> MTYKYNCCDDGSGTTVGSVVRFDNVTLLIDPGWNPSKVSYEQCIKYWEKVIPEIDVIILSQPTIECLGAHSLLYYNFTSHFISRIQVYATLPVINLGRVSTIDSYASAGVIGPYDTNKLDLEDIEISFDHIVPLKYSQLVDLRSRYDGLTLLAYNAGVCPGGSIWCISTYSEKLVYAKRWNHTRDNILNAASILDATGKPLSTLMRPSAIITTLDRFGSSQPFKKRSKIFKDTLKKGLSSDGSVIIPVDMSGKFLDLFTQVHELLFESTKINAHTQVPVLILSYARGRTLTYAKSMLEWLSPSLLKTWENRNNTSPFEIGSRIKIIAPNELSKYPGSKICFVSEVGALINEVIIKVGNSEKTTLILTKPSFECASSLDKILEIVEQDERNWKTFPEDGKSFLCDNYISIDTIKEEPLSKEETEAFKVQLKEKKRDRNKKILLVKRESKKLANGNAIIDDTNGERAMRNQDILVENVNGVPPIDHIMGGDEDDDEEEENDNLLNLLKDNSEKSAAKKNTEVPVDIIIQPSAASKHKMFPFNPAKIKKDDYGTVVDFTMFLPDDSDNVNQNSRKRPLKDGAKTTSPVNEEDNKNEEEDGYNMSDPISKRSKHRASRYSGFSGTGEAENFDNLDYLKIDKTLSKRTISTVNVQLKCSVVILNLQSLVDQRSASIIWPSLKSRKIVLSAPKQIQNEEITAKLIKKNIEVVNMPLNKIVE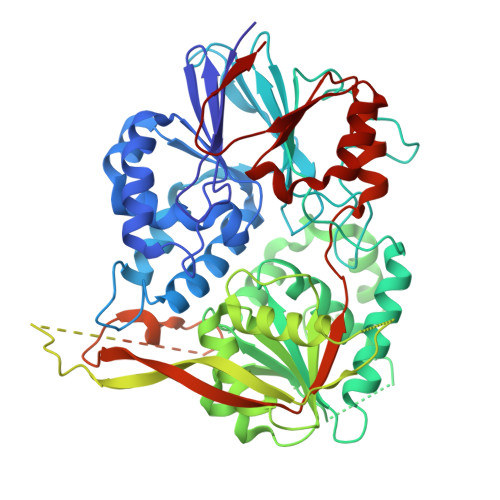FS(3~{R},4~{S},5~{R},6~{S},7~{S},9~{S},11~{R},12~{S},13~{R},14~{R})-3,5,7,9,11,13,14-heptamethyl-4,6,12-tris(oxidanyl)-1-oxacyclotetradecane-2,10-dione 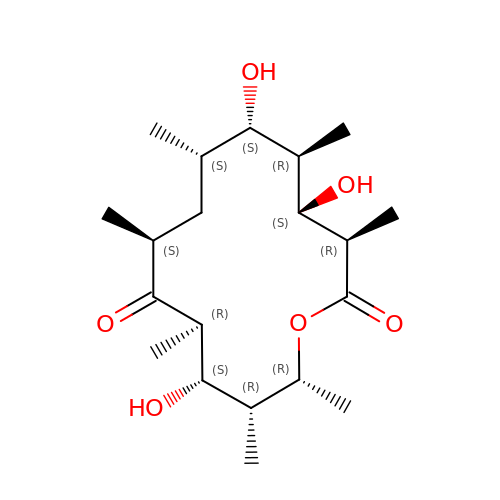| C20 H36 O6 | OLPAVFVRSHWADO-ODNSKKOKSA-N>GSKNLIGRHLRLGSVESQPFMFFATEGCEGNDCWSGMVNDMVVKLSEDLGFTYEYI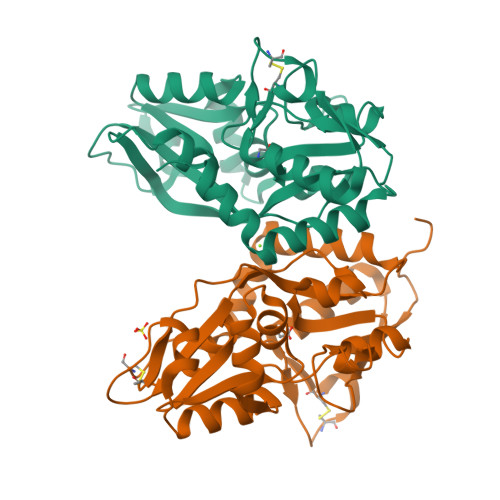QPDDRKFGALNKTTNEWNGMIRDLLDDKTDMIAIDLSTNSARKSAIDYSFPFMDAGIKAVVKGEGTTLNQVLELLDQDKYKWGVIGSRHPETLLKTHRDSRYSRLVDEGVELKDLNHAIETLRGGLFVFIDEGPVLAHNLISDCDVFSVGEEFQSFEYAFGLPKDSPYKSLIDSHLLKFREEGFIDILWEKWSSGNSVCS[2x]>SNAGKMFIGGLSWQTSPDSLRDYFSKFGEIRECMVMRDPTTKRSRGFGFVTFADPASVDKVLGQPHHELDSKTIDPKV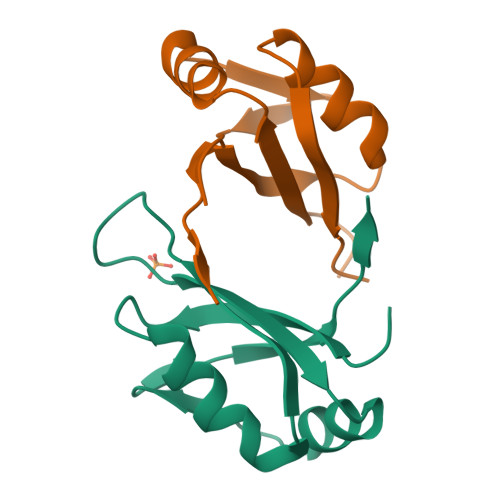AFPRRAQPKMVTRTKK[2x]In Gram-positive Firmicutes, it also has a role in natural transformation, while in Gram-negative bacteria, ComM is the canonical transformation-specific helicase. Comprehensive biochemical characterization of RadA from Escherichia coli, S. pneumoniae, B. subtilis and Thermus thermophilus and ComM from V. cholerae revealed that they are functional homologs during HR. Both RadA and ComM were found to be ring-shaped hexameric DNA motors powered by ATP hydrolysis to direct three-stranded DNA branch migration in vitro. Here, we present and compare the cryoEM (cryogenic electron microscopy) structures of RadA and ComM from S. pneumoniae and Legionella pneumophila, respectively, in interaction with DNA.

Local refinements were also carried out on half of the hexamer and the Lon domain, resulting in an improvement in the quality of the map in these regions. The final atomic model of the ComM protomer reveals that the N-terminal domain comprises a Lon protease-like domain, as deduced from its sequence. Despite their low sequence identity (28%), the two Lon domains superimpose with a root mean square deviation (RMSD) of only 1 Å. In ComM, there are electrostatic interactions between S26 and R50 as well as E22 and R117. In contrast to traditional Lon proteases, the interior of the Lon domain ring is rich in basic residues, consistent with potential DNA coordination at the center of the pore. This is further supported by the observation that ComM interacts with DNA via three lysines, K43, K46, and K64, which form hydrogen bonds with the DNA backbone within the central pore. Indeed, the Lon domain of ComM contacts DNA in at least three positions: K43, K46 and K64. In contrast, we show that ComM has a larger pore radius with a diameter of 24 Å. Conversely, the p-value for ComM, which is close to 0.5, reflects a non-specific interaction and is similar to the average value for its structure. These findings suggest that the hexamerization of ComM, which is dependent of DNA and ATP, is primarily driven by global solvation-free energy rather than by interactions between specific residues within the Lon domain.

>[6x]MSLAFTKTRSTIGIVAQPVSVEVHLSNGLPSFTMVGLAETAVKESKDRVRSAIINSQFEFPCRKITVNLGPANLPKTGSGFDLPIALGILAASEQIPLTNLANHEFIGELALSGELRGVSAIIPAVLAAHKDNQHLIIANANAAEASLTGHQKVFTANNLREVCDYLCQGTSLQSLPPKPDLLLNNYELDWSDIKGQQHAKNAMVIAACGGHSILLSGAPGSGKTMMAKRFSTLLPELSETQALECAAINSIRGKLPDFREWRLPPFRAPHHTASPVALVGGGNPPKPGEISLAHHGVLFLDELPEFNRQVLETLREPLESGHICISRAAAQIEFPAKFQLIAAMNPCPCGQWGNSQANCMCTPDRISRYLAKLSAPLLDRIDMQVTIHALSQEELIKPNTHLEKQSLAIREKVTKMHEIQMARQDSLNANLNSKTCEMVCELGSEEQLFLREVMSKLKLSARGYHRLLKVSRTIADMNSSKKVLLNHLQQALSYKQNLHLPKHHHHHH>[4x]MALRFEALYPEGMCPGWSVVVKGKTSSNTSMFEINFLSHPGDQIAFHFNPRFASSRIVCNSFLANHWGKEEVNKTFPFEAKEPFQVEIYSDQDYFHIFIDEN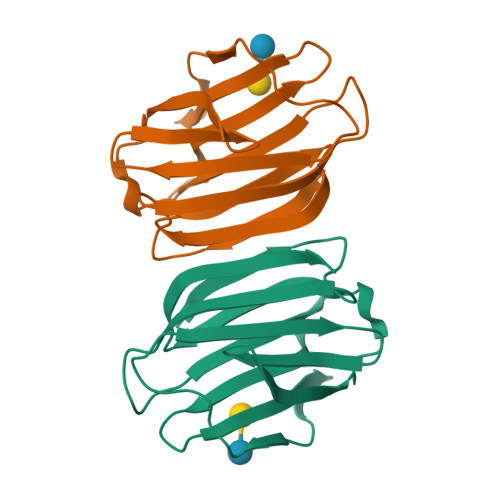KILQYKHRQKQLSSITKLQILNDIEISSVEITKRGLY2-[[2,6-bis(chloranyl)-3-phenylmethoxy-phenyl]amino]pyridine-3-carboxylic acid | C19 H14 Cl2 N2 O3 | 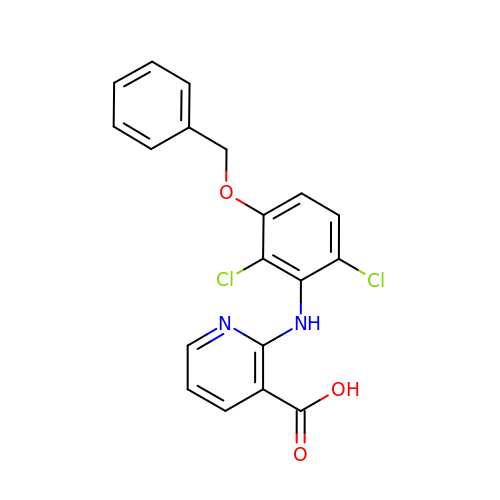AYGDOYFDJDUPSS-UHFFFAOYSA-N>[4x]SEKEKVEELAQRIREQLPDTELAREAQELADEARKSDDSEALKVVYLALRIVQQLPDTELAREALELAKEAVKSTDSEALKVVYLALRIVQQLPDTELARLALELAKKAVEMTAQEVLEIARAALKAAQAFPNTELAELMLRLAEVAARVMKELERNDEEIKKSDELDDESLLEDIVELLKEIIKLWKILVEVSDVMLKLIS;>[4x]GPVDEIDKEVKKLEEEAKKSQEEVERLKQEVEKASKAGLDHEGDSRIFKKIHDVVTKQIKVILRLIAVYAELVAIIG;>[4x]GSKQKEAIKVYLELLEVHSRVLKALIEQIKLFIELIKRPDEDLADKVRKSSEELKKIIKEVEKILRKVDDILYKVKS

We designed helical heterotrimers with specificity conferred by buried hydrogen bond networks and large aromatic residues to enhance shape complementary packing. Crystal structures of a helical bundle heterotrimer and extended versions, with helical repeat proteins fused to individual subunits, showed all three chains assembling in the designed orientation. We succeeded in determining three high-resolution structures for DHT03: the original base construct, a one-arm version (1arm_A21/B/C) and an elongated two-arm version (2arm_A21/B21/C long). We show that computational design can create cooperative ABC heterotrimers that can assemble as free-standing helical units or as hubs in larger designed assemblies.

Ten one-arm fusions to DHT03 were tested via tricistronic expression, with two eluting with monodisperse peaks by SEC and forming exclusive ABC heterotrimers by nMS (rows 1 and 2). Over the core heterotrimer in both structures, the backbones are very similar to that of the base heterotrimer crystal structure, but the resolution is not high enough to determine the state of the designed hydrogen bond networks. The designed junctions between the repeat protein arms and the core bundle are recapitulated in the crystal structures and hold the repeat arms rigidly in close to the designed orientations. Deviations between the crystal structure and design model in the repeat protein arms increase with increasing distance from the central bundle due to lever arm effects arising from the compounding of small orientational differences in the structures of the individual repeats. These structures show that the DHTs can serve as rigid interaction hubs in asymmetric assemblies, which have been more difficult to design than symmetric ones.> TDSLSFSFINFDRDERNLIFQGDAHTSRNNILQLTRTDSNGAPVRSTVGRILHSAQVRLWEKSTNRVANFQTQFSFFLSSPLSNPADGIAFFIAPPDTTIPSGSAGGLLGLFNPRTALNESANQVLAVEFDTFFAQNSNTWDPNYQHIGIDVNSIRSSKVVRWERREGKTLNVLVTYNPSTRTIDVVATYPDGQRYQLSHVVDLTTILPEWVRVGFSA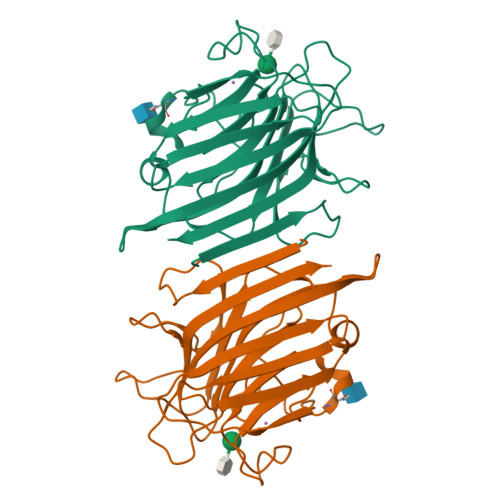ASGEQFQTHNLESWSFTSTLL> GHMNSFVGLRVVAKWSSNGYFYSGKITRDVGAGKYKLLFDDGYECDVLGKDILLCDPIPLDTEVTALSEDEYF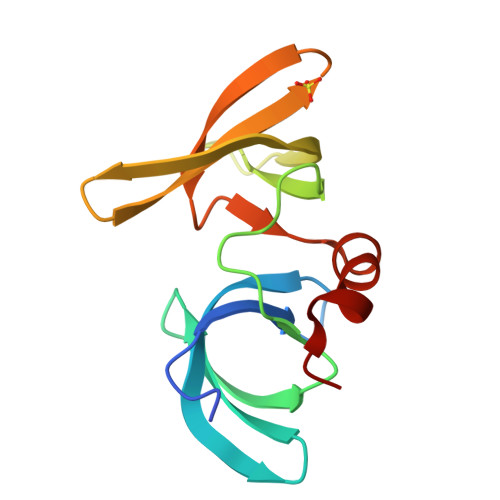SAGVVKGHRKESGELYYSIEKEGQRKWYKRMAVILSLEQGNRLREQYGLG>[2x]GHHHHHHAMSMQDTLLTLDTPAAVIDLDRMQRNIARMQQRMDAQGVRLRPHVKTSKSVPVAAAQRAAGASGITVSTLKEAEQFFAAGTTDILYAVSMAPHRLPQALQLRRRGCDLKLIVDSVAAAQAIAAFGREQGEAFEVWIEIDTDGHRSGVGADDTPLLLAIGRTLHDGGMRLGGVLTHAGSSYELDTPEALQALAERERAGCVQA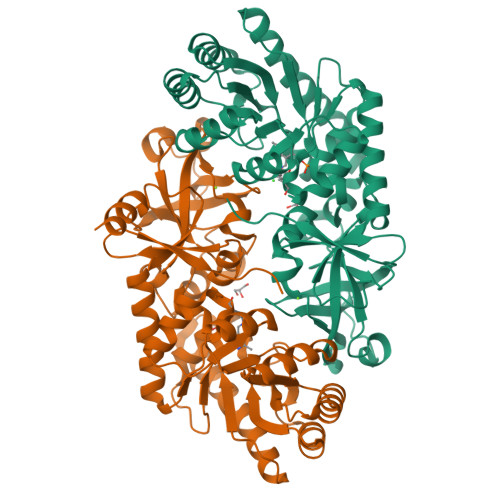AEALRAAGLPCPVVSVGSTPTALAASRLDGVTEVRAGVYVFFDLVMRNIGVCAAEDVALSVLATVIGHQADKGWAIVDAGWMAMSRDRGTARQKQDFGYGQVCDLQGRVMPGFVLTGANQEHGILARADGAAEADIATRFPLGTRLRILPNHACATGAQFPAYQALAADGSVQTWERLHGW> MGFIGNSLPMQAVYRVIESAASSKATVFITGESGTGKEVCAEAIHAASPRHDKPFIALNCAAIPKDLIESELFGHVKGAFTGASTERQ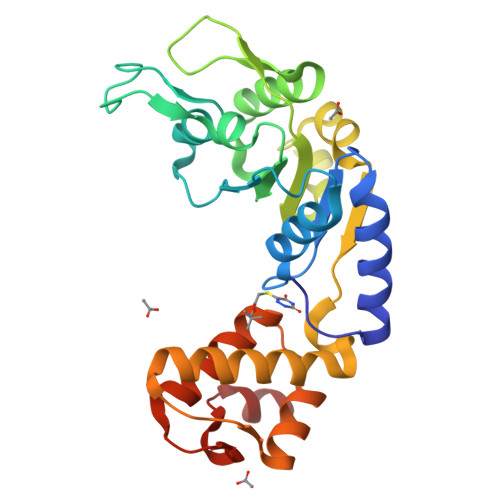GAVEMAHNGTLMLDELCEMDLDLQSKLLRFIQTGTYQKVGSSKMSSVDVRFVCATNRNPWEEVQEGRFREDLYYRLHVIPISLPPLRERGGDIIEIAHALLGLMSLEEGKSFSRFSEPVLRLFESYSWPGNVRELQNVIRNIVVLNTDDEVKLEMVPPPILEHHHHHH> MADFARSLSITTPEEMIEKAKGETAYLPCKFTLSPEDQGPLDIEWLISP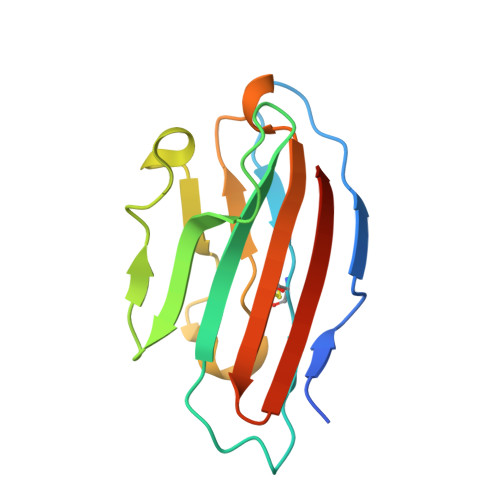ADNQKVDQVIILYSGDKIYDDYYPDLKGRVHFTSNDLKSGDASINVTNLQLSDIGTYQCKVKKAPGVANKKIHLVVLVK> SPSESLITQKQIMSQAGSTGSNSGLGSITDLLNNILSVANQIIYNSAVALPLQLDTLESTLLTAIKSLQTSDKLEQNCSWSAALINDNRYINGINQFYFSIAEGRNLTLGPLLNMPSFIPTATTPEGCTRIPSFSLTKTHWCYTHNVILNGCQDHVSSNQFVSMGIIEPTSAGFPFFRTLKTLYLSDG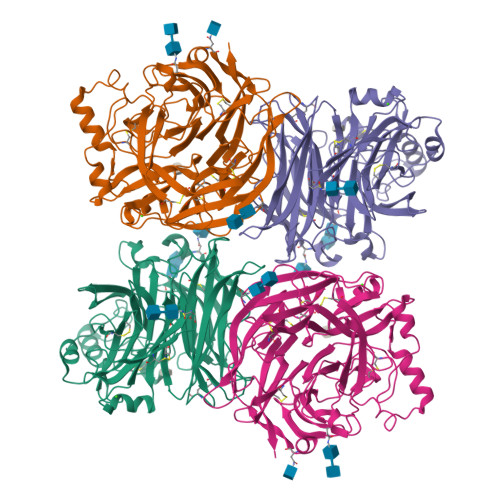VNRKSCSISTVPGGCMMYCFVSTQPERDDYFSAAPPEQRIIIMYYNDTIVERIINPPGVLDVWATLNPGTGSGVYYLGWVLFPIYGGVIKGTSLWNNQANKYFIPQMVAALCSQNQATQVQNAKSSYYSSWFGNRMIQSGILACPLRQDLTNECLVLPFSNDQVLMGAEGRLYMYGDSVYYYQRSNSWWPMTMLYKVTITFTNGQPSAISAQNVPTQQVPRPGTGDCSATNRCPGFCLTGVYADAWLLTNPSSTSTFGSEATFTGSYLNTATQRINPTMYIANNTQIISSQQFGSSGQEAAYGHTTCFRDTGSVMVYCIYIIELSSSLLGQFQIVPFIRQVTLS> MVQAMERPSSAKLPPLDHPLADIIYRLEAGGALIPDTPVNLMKIIGMYKAYSIPMDFYWRDLLYLGERVFINPFPFFKYFPTKEYFELPNHYAGDTADLRIWRGPAHAHPELMEFIEKGETGKMPRLLHHLWHDRI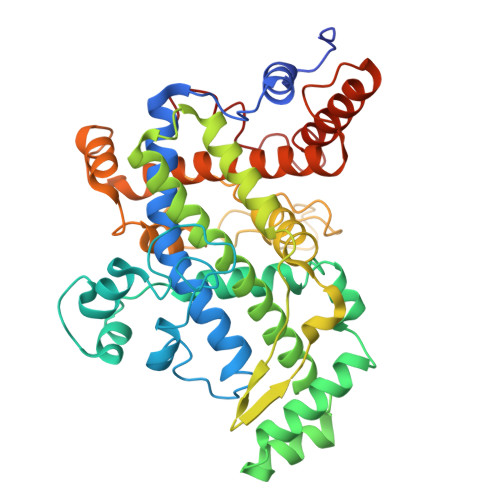NMEFSEDLARAMMWHRMGGQLDIYLDSEEYKAAADKAIRAYFKRNPLMLGLYKLFPDLFLEQARQATYMNVLGLFWEVMAPVFFEISDRYDEGSITSVKDAMNFLVNGIFAIAGRPIYHHVYIDDEVHVLVPKEKGFMWLYEAAFPYVEAVFYRTSPFRGTKSYNAQANQVPTDQVDFHYGILFADKFPVGTAGIPPTLLHQDMYHFLPQYLKDYFHQHCRGEDDILVQLGIAFQHAMYTVTSAVLQATRAAFYYPLDDPNPEHLMANRRFFVAQMDRFLRPQYGIAEACKIRNVQDPNYL> SIWGLVNEEDAEIDEDDLSKQEDGGEQPLRKVRTLAQSKPSDKEVILKTDGTFGTLSGKDDSIVEEKAYEPDLSDADFEGIEASPKLDVSKDWVEQLILAGSSLRSVFATSKEFDGPCQNEIDLLFSECNDEIDNAKLIMKERRFTASYTFAKFSTGSMLLTKDIVGKSGVSIKRLPTELQRKFLFDDVYLDKEIEKVTIEARKSNPYPQISESSLLFKDALDYMEKTSSDYNLWKLSSILFDPVSYPYKTDNDQVKMALLKKERHCRLTSWIVSQIGPEIEEKIRNSSNEIEQIFLYLLLNDVVRASKLAIESKNGHLSVLISYLGSNDPRIRDLAELQLQKWSTGG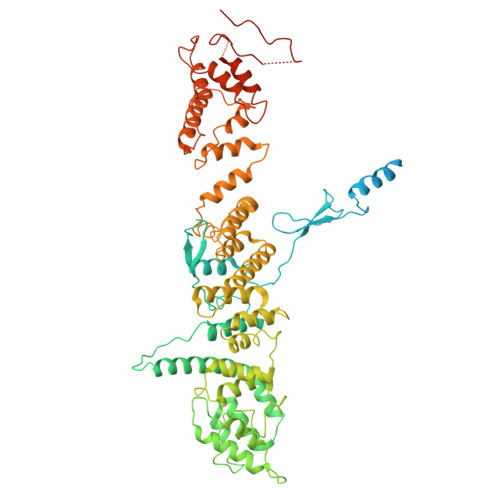CSIDKNISKIYKLLSGSPFEGLFSLKELESEFSWLCLLNLTLCYGQIDEYSLESLVQSHLDKFSLPYDDPIGVIFQLYAANENTEKLYKEVRQRTNALDVQFCWYLIQTLRFNGTRVFSKETSDEATFAFAAQLEFAQLHGHSLFVSCFLNDDKAAEDTIKRLVMREITLLRASTNDHILNRLKIPSQLIFNAQALKDRYEGNYLSEVQNLLLGSSYDLAEMAIVTSLGPRLLLSNNPVQNNELKTLREILNEFPDSERDKWSVSINVFEVYLKLVLDNVETQETIDSLISGMKIFYDQYKHCREVAACCNVMSQEIVSKILEKNNPSIGDSKAKLLELPLGQPEKAYLRGEFAQDLMKCTYKI> MRGSHHHHHHGMASMSSEKLFRIQ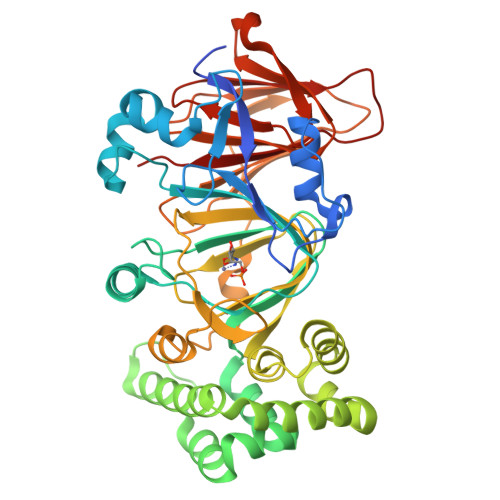CGYQNYDWGKIGSSSAVAQFVHNSDPSITIDETKPYAELWMGTHPSVPSKAIDLNNQTLRDLVTAKPQEYLGESIITKFGSSKELPFLFKVLSIEKVLSIQAHPDKKLGAQLHAADPKNYPDDNHKPEMAIAVTDFEGFCGFKPLDQLAKTLATVPELNEIIGQELVDEFISGIKLPAEVGSQDDVNNRKLLQKVFGKLMNTDDDVIKQQTAKLLERTDREPQVFKDIDSRLPELIQRLNKQFPNDIGLFCGCLLLNHVGLNKGEAMFLQAKDPHAYISGDIIECMAASDNVVRAGFTPKFKDVKNLVEMLTYSYESVEKQKMPLQEFPRSKGDAVKSVLYDPPIAEFSVLQTIFDKSKGGKQVIEGLNGPSIVIATNGKGTIQITGDDSTKQKIDTGYVFFVAPGSSIELTADSANQDQDFTTYRAFVEA> MTSRKKVLLKVIILGDSGVGKTSLMNQYVNKKFSNQYKATIGADFLTKEVMVDDRLVTMQIWDTAGQERFQSLG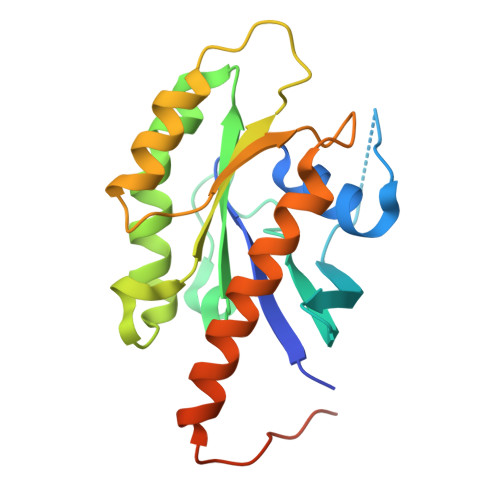VAFYRGADCCVLVFDVTAPNTFKTLDSWRDEFLIQASPRDPENFPFVVLGNKIDLENRQVATKRAQAWCYSKNNIPYFETSAKEAINVEQAFQTIARNALKQETEVELYNEFPEPIKLDKNERAKASAESCSC> AKPAQGAKYRGSIHDFPGFDPNQDAEALYTAMKGFGSDKEAILDIITSRSNRQRQEVCQSYKSLYGKDLIADLKYELTGKFERLIVGLMRPPAYCDAKEIKDAISGIGTDEKCLIEILASRTNEQMHQLVAAYKDAYERDLEADIIGDTSGHFQKMLVVLLQGTREEDDVVSEDLVQQDVQDLYEAGELKWGTDEAQFIYILGNRSKQHLRLVFDEYLKTTGKPIEASIRGELSGDFEKLMLAVVKCIRSTPEYFAERLFKAMKGLGTRDNTLIRIMVSRSELDMLDIREIFRTKYEKSLYSMIKNDTSGEYKKTLLKLSGGDDDAAGQFFPEAAQVAYQMWELSAVARVELKGDVRPANDFNPDADAKALRKAMKGLGTDEDTIIDIITHRSNVQRQQIRQTFKSHFGRD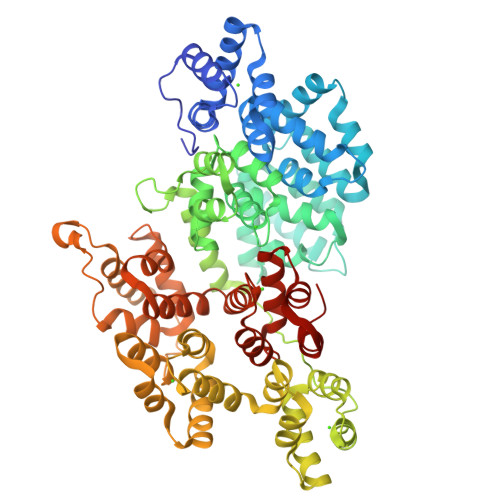LMTDLKSEISGDLARLILGLMMPPAHYDAKQLKKAMEGAGTDEKALIEILATRTNAEIRAINEAYKEDYHKSLEDALSSDTSGHFRRILISLATGHREEGGENLDQAREDAQVAAEILEIADTPSGDKTSLETRFMTILCTRSYPHLRRVFQEFIKMTNYDVEHTIKKEMSGDVRDAFVAIVQSVKNKPLFFADKLYKSMKGAGTDDKTLTRIMVSRSEIDLLNIRREFIEKYDKSLHQAIEGDTSGDFLKALLALCGGED Here we characterize the structure and function of p43, the single most abundant protein in secretions from adult T. muris, whipworm. Structural determination by X-ray crystallography reveals potential interaction with glycosaminoglycans and the host cytokine IL-13. Binding studies confirm high-affinity binding to heparan sulfate (HS) and IL-13. Moreover, p43 inhibits IL-13 immune function both in vitro and in vivo.

Trichuris muris p43 comprises 397 amino acids (AA), 36 cysteine residues (9%), and a histidine-rich C-terminal region (45% of terminal 29 residues are His). Analyses of the primary sequence reveal an internal repeat with residues 1–180 and 181–394 sharing 34% amino acid sequence identity. The protein has mixed α and β composition with 16 β-strands and 6 α-helices. The crystal structure reveals contiguous electron density for residues 21–368, and no electron density is observed for the histidine-rich C-terminal region. The structure shows that all 36 of the available cysteine residues are involved in the formation of 18 intramolecular disulfide bonds. In each of the two domain repeats, eight disulfides are conserved, while the bond between C274 and C277 has no equivalent in domain 1 and C131 from domain 1 bonds to C362 of domain 2. The disulfide bonding pattern is unevenly distributed throughout the protein clustering around the β-sandwich region (β4–β8). There are three potential N-glycosylation sites predicted at positions 57, 174, and 287, and the crystal structure shows clear evidence of glycosylation at residues 57 and 287, but not at position 174. Surface representation of p43 by electrostatic surface potential indicates a negatively charged region, suggestive of a possible binding cleft between the two domain repeats. Native mass spectrometry and collision-induced dissociation (CID) experiments showed p43-bound IL-13 with a 1:1 stoichiometry and confirmed that p43 was a flexible molecule with the potential for conformational change upon activation.

>[2x]MLVLFFPLLLTVGLSTAGHVKCPDFGDWKPWTDCLWYPPQHMYSKLSHACGMHAHRNLTGVMDLPHGHKTPPPCGHCSFKFRCRRRPNTEGCYPLDGEVEVCHDHSDICTLPKLPHLGCGYAFINEKLKQCFTRPDTPSYVRLGYRKMFESIPKKHCIEKDGMCKCCCGDYEPNESGTECIKPPAHDCPAYGPPSEWSECLWFPLKNIVSHVYDHCHVHKEPDGYEPHSVAPANVHIPEKCGFCSFRVKCMKRDKKDGCFPLKLGKKSCGKDDCPTCGDICTLDKINGSCAFPRVMKEKIWDDFTATSKEKHMPHWKRDGYAKMLMQLPYSNCKEVGDKCKCCCHPYEPNKDGTACVVKEYCKRVHELHHHDHHGHGEEHHKSSSSESKEHHHH> MDRLSRLRQMAAENQPAEASDAAGGAEAQIEETSLSAQPEPFMADFFNRVKRIRDNIEDIEQAIEQVAQLHTESLVAVSKEDRDRLNEKLQDTMARISALGNKIRADLKQIEKENKRAQQEGTFEDGTVSTDLRIRQSQHSSLSRKFVKVMTRYNDVQAENKRRYGENVARQCRVVEPSLSDDAIQKVI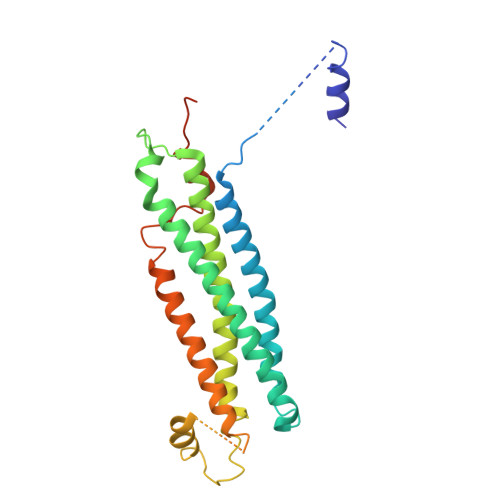EHGTEGIFSGMRLEGAEAKLNEIRDRHKDIQQLERSLLELHEMFTDMSTLVASQGEMIDRIEFSVEQSHNYVKKATEQVVQARHYQESAR> MKVWLVGAYGIVSTTAMVGARAIERGIAPKIGLVSELPHFEGIEKYAPFSFEFGGHEIRLLSNAYEAAKEHWELNRHFDREILEAVKSDLEGIVARKGTALNCGSGIKELGDIKTLEGEGLSLAEMVSRIEEDIKSFADDETVVINVASTEPLPNYSEEYHGSLEGFERMIDEDRKEYASASMLYAYAALKLGLPYANFTPSPGSAIPALKELAEKKGVPHAGNDGKTGETLVKTTLAPMFAYRNMEVVGWMSYNILGDYD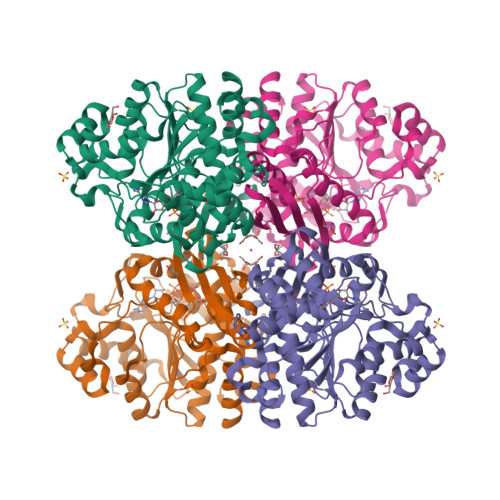GKVLSARDNKESKVLSKDKVLEKMLGYSPYSITEIQYFPSLVDNKTAFDFVHFKGFLGKLMKFYFIWDAIDAIVAAPLILDIARFLLFAKKKGVKGVVKEMAFFFASPMDTNVINTHEQFVVLKEWYSNLK>VHPITYYPVDTQRLVRSNAERIRHKPYAHYFNPDVAVPEEVFAALKAPLEPEQVLGTSSTELNRL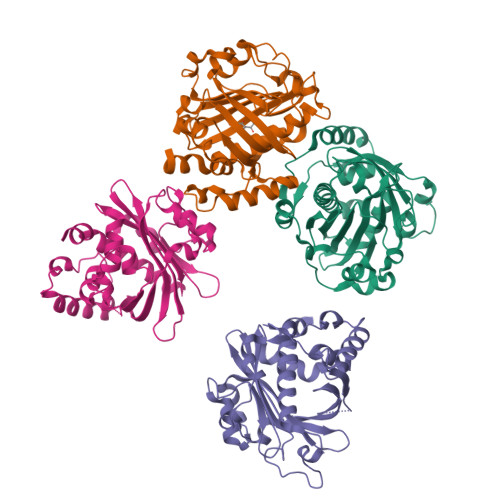LEPGYLEGETGYCGLPDGAGYTSSLVRFPGATPEMFRWWFWWHSFEPERYSLWHPWCHADIWRTDPETETAPNLTDEQRYVGSTHHINEYIGQDPLDIEITFIDPARWGFDADGFAAAGIGAHACGSVLMKGSHMRLATMVHLARITDDGFELRSRYWIADRAEPRHDPVAGIAQLTTVPGFSGERQAYEQLVHDQTEFNHLATFLPDIYQEFG[4x]> TPATQPLINAEPAVAAQTEQNPQVGQVMPGVQGADAPVVAQNGPSRDVKLTFAQIAPPPGSMVLRGINPNGSIEFGMRSDEVVTKAMLNLEYTPSPSLLPVQSQLKVYLNDELMGVLPVTKEQLGKKTLAQMPINPLFITDFNRVRLEFVGHYQDVCENPASTTLWLDVGRSSGLDLTYQTLNVKNDLSHFPVPFFDPRDNRTNTLPMVFAGAPDVGLQQASAIVASWFGSRSGWRGQNFPVLYNQLPDRNAIVFATNDKRPDFLRDHPAVKAPVIEMINHPQNPYVKLLVVFGRDDKDLLQAAKGIAQGNILFRG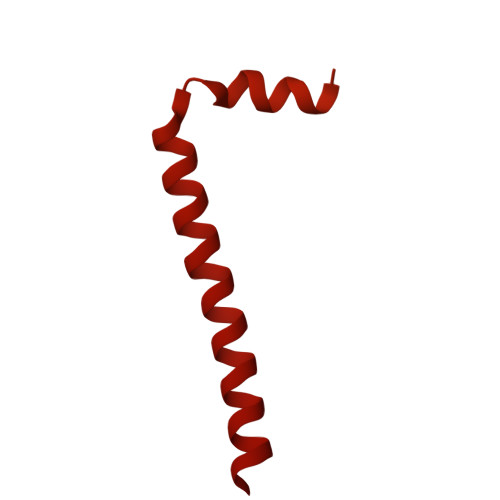ESVVVNEVKPLLPRKPYDAPNWVRTDRPVTFGELKTYEEQLQSSGLEPAAINVSLNLPPDLYLMRSTGIDMDINYRYTMPPVKDSSRMDISLNNQFLQSFNLSSKQEANRLLLRIPVLQGLLDGKTDVSIPALKLGATNQLRFDFEYMNPMPGGSVDNCITFQPVQNHVVIGDDSTIDFSKYYHFIPMPDLRAFANAGFPFSRMADLSQTITVMPKAPNEAQMETLLNTVGFIGAQTGFPAINLTVTDDGSTIQGKDADIMIIGGIPDKLKDDKQIDLLVQATESWVKTPMRQTPFPGIVPDESDRAAETRSTLTSSGAMAAVIGFQSPYNDQRSVIALLADSPRGYEMLNDAVNDSGKRATMFGSVAVIRESGINSLRVGDVYYVGHLPWFERLWYALANHPILLAVLAAISVILLAWVLWRLLRIISRRRLNPDNE> SMKIPNIGNVMNKFEILGVVGEGAYGVVLKCRHKETHEIVAIKKFKDSEENEEVKETTLRELKMLRTLKQEN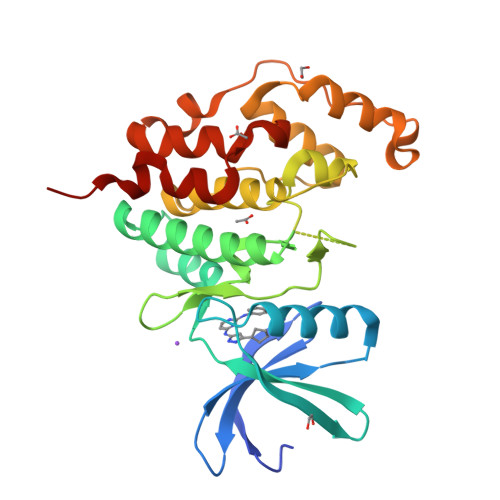IVELKEAFRRRGKLYLVFEYVEKNMLELLEEMPNGVPPEKVKSYIYQLIKAIHWCHKNDIVHRDIKPENLLISHNDVLKLCDFGFARNLSEGNNANYDEEVATRWYRSPELLLGAPYGKSVDMWSVGCILGELSDGQPLFPGESEIDQLFTIQKVLGPLPSEQMKLFYSNPRFHGLRFPAVNHPQSLERRYLGILNSVLLDLMKNLLKLDPADRYLTEQCLNHPTFQTQRLL3,5,6,7-TETRAHYDROXY-2-(3,4-DIHYDROXYPHENYL)-4H-CHROMEN-4-ONE 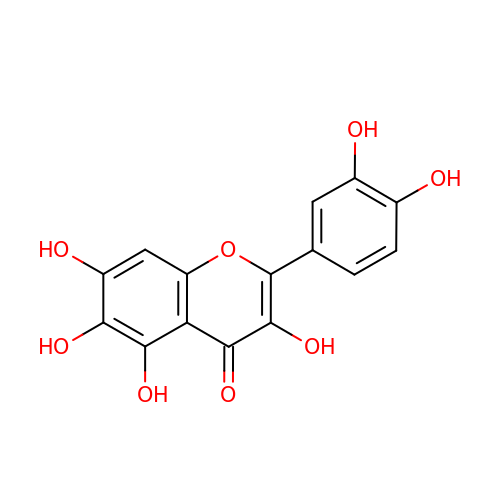| C15 H10 O8 | ZVOLCUVKHLEPEV-UHFFFAOYSA-N>[2x]LKQVRPGMDLSKVVLPTFILEPRSFLDKLSDYYYHADFLSEAALEENPYFRLKKVVKWYLSGFYKKPKGLKKPYNPILGETFRCLWIHPRTNSKTFYIAEQVSHHPPISAFYVSNRKDGFCLSGSILAKSKFYGNSLSAILEGEARLTFLNRGEDYVMTMPYAHCKGILYGTMTLELGGTVNITCQKTGYSAILEFKLKPFLGSSDCVNQISGKLKLGKEVLATLEGHWDSEVFITDKKTDNSEVFWNPTPDIKQWRLIRHTVKFEEQGDFESEKLWQRVTRAINAKDQTEATQEKYVLEEAQRQAARDRKTKNEEWSCKLFELDPLTGEWHYKFADTRPWDPLNDMIQFEKDGVIQTKVKHRTPMVSVPKMKHKPTRQQK

Lipid transfer at membrane contact sites, such as the ER–plasma membrane contact site, is facilitated by oxysterol-binding protein (OSBP)-related proteins (ORPs). Most human ORP proteins contain an N-terminal pleckstrin homology (PH) domain and a C-terminal lipid transport domain. The PH domain recognizes and binds the target membrane, while the C-terminal transmembrane helix anchors ORP8 to the donor (ER) membrane. In the case of ORP8, the cargo lipid is phosphatidylserine (PS), which is synthesized in the ER but needs to be transported to the plasma membrane.

However, despite years of efforts, we have only been successful in elucidating the structure of unliganded ORD8. The structure was solved by molecular replacement using an AlphaFold model. The RMSD between the model and the refined crystal structure was 1.44 Å, and the structure fitted the 2mFo-DFc composite omit map well. The overall fold is reminiscent of a β-barrel composed of anti-parallel β-strands. Compared to the well-studied β-barrel structure, the GFP, the ORD8 domain is composed of more β-strands (19 in total), whereas GFP is composed of 11 β-strands. However, in the case of ORD8, in one side of this β-barrel, the β-strands are replaced by three α-helices. The fold is therefore actually a mixture of alpha and beta. This observation is consistent with the previously reported structures of ORP2 and ORP3 that exhibit similar fold with RMSDs at 5.27 Å and 5.32 Å, respectively. The structure also revealed a rather large cavity (its volume was estimated using spaceball to be approximately 1860 Å3) in the middle of the barrel. This cavity, consistently with the previously reported structure of Osh6, represents the lipid-binding site. The full-length (including the lid) ORD domain never produced any crystals.> MSSIINKEVQEAPLKWVKNWSDEEIKALVDEEKGLLDPRIFSDQDLYEIELERVFARSWLLLGHEGHIPKAGDYLTTYMGEDPVIVVRQKDRSIKVFLNQCRHRGMRIERSDFGNAKSFTCTYHGWAYDTAGNLVNVPYEKEAFCDKKEGDCGFDKADWGPLQARVDTY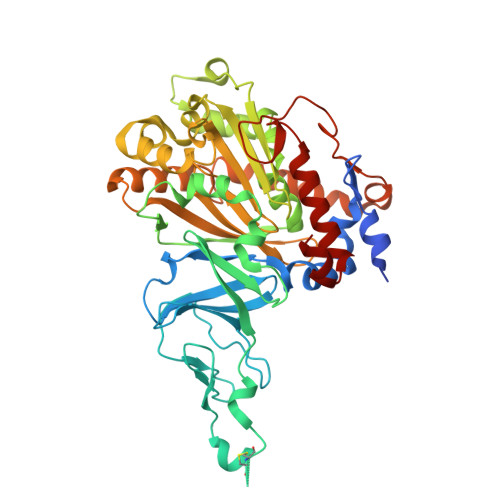KGLIFANWDTEAPDLKTYLSDATPYMDVMLDRTEAVTQVITGMQKTVIPCNWKFAAEQFCSDMYHAGTMAHLSGVLSSLPPEMDLSQVKLPSSGNQFRAKWGGHGTGWFNDDFALLQAIMGPKVVDYWTKGPAAERAKERLGKVLPADRMVAQHMTIFPTCSFLPGINTVRTWHPRGPNEIEVWSFIVVDADAPEDIKEEYRRKNIFTFNQGGTYEQDDGENWVEVQRGLRGYKARSRPLCAQMGAGVPNKNNPEFPGKTSYVYSEEAARGFYHHWSRMMSEPSWDTLKS>MADGGESSNANAGEGTSGGGGSGPLALTGGSRAGGTIGGGGAGSVGFSTGGWTAGTYFSDNKVVTNQTRQFLTPIYNGHTYKALQADDLTNENDKSKWNGITTPWGYFNFNCYASHFSPQDWQRMCNEYKRWRPKRLRVQIYNLQLKTIQSNGADTQYNNDLTAAVHILVDGSHQFPWAQHPWDDTCAPELPYVIYKTPQYAYFQNLAGLANNVGTNSANKFLKMNTPLYVLETMSHEVLRTGEDTSFEFEMSSGWVDNQTNFCPPQLDFNPLHDTRRVAPRATNNTTQYAPYPKFKKPSNWVPGPGMAYPGRGEADGKRPAPMTVTLRPNTFIDAGNNTTDRFQQASYQEWKPTDDTIIGQSINVGPINCAATDPDAVTTAADAEDDVANPNTDKVSSHRYSIDMTRWNAIQINVRRNNGTPETTQIYRHYLYPMQAWNSNQIDRYTPIWDKVPNTEWHTMLASSDGTLPMTHPPGTIFIKCSKIPVPSENNADSYLNIYCTGQVSYEIEWECERYNTKNWRPELRVDPKNWTDPNNYNLNTQGGYIVNEELYETMPTKIGINRVN[60x]

To expand the structural repertoire of determined capsid structures for the diverse Bocaparvovirus genus, viruses infecting dogs (CnMV), pigs (PBoV1), and rats (RBoV) were selected. The ORFs of these viruses coding for the major capsid protein VP2 were cloned into the pFastBac1 plasmid to enable the production of the virus-like particles (VLPs), using the Bac-to-Bac expression system in insect Sf9 cells. In the icosahedral capsid, the 60 VPs assemble via two-, three-, and fivefold symmetry-related VP interactions, resulting in pores at the fivefold symmetry axes, protrusions surrounding the threefold axes, and depressions at the twofold axes.

In 2017, rat bocavirus (RBoV) was identified from brown rats in China. As a recent addition to the Bocaparvovirus genus, its pathogenicity is still unknown, but has been shown to have broad tissue tropism. Its capsid (VP1) amino acid sequence identity is 37% and 41% for BPV and HBoV1, respectively. Following cryo-EM data collection, three-dimensional-image reconstruction of the capsids, utilizing 50,866 (CnMV), 98,388 (PBoV1), and 9199 (RBoV) individual capsid images, resulted in a resolution of 2.72, 2.31, and 2.52 Å, respectively. In the case of PBoV1 and RBoV, the cryo-EM maps for the most part also showed densities for the carbonyl groups of the main-chain and densities for a specific rotamer for the individual amino acids, guiding the model building for these viruses. Capsid structures previously determined for the Bocaparvovirus genus showed disperse protrusions surrounding the threefold axis that do not significantly extend radially from the capsid surface. In contrast, the CnMV capsid shows very prominent threefold protrusions, while PBoV1 and RBoV follow the previously described characteristics of the genus. In PBoV1 and RBoV, the shorter VR-III does not cover the entire twofold region, but their loop also advances the twofold axis and restricts the size of the depression. Additionally, a different loop confirmation of VR-IX in CnMV, PBoV1, and RBoV compared to HBoV1 and BPV near the twofold axis further causes an increase in the radial capsid surface in this region. Another feature previously observed for the bocaviruses, with the exception of GBoV1, was the presence of density extending into the interior of the capsid below the fivefold channel. This density was also seen for CnMV, but is absent in the PBoV1 and RBoV capsids.>FQAMAITQKRPVYLQLVDRIKNEVATDVLSANDQLPSVRETALQEKINPNTV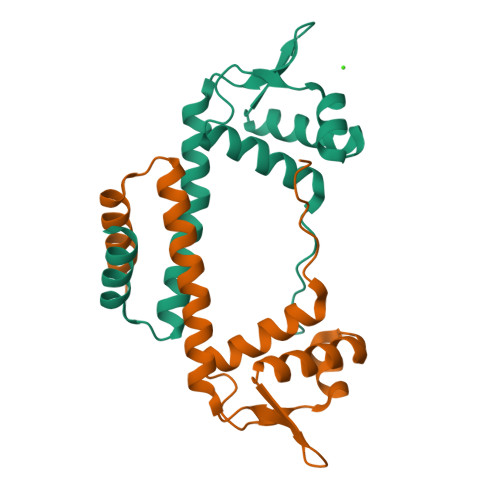AKAYKELEAQKVIRTIPGKGTFITGNTASVKNSNQNRLLADLSQVIAELIKSGVKGERIKKIVNDILGGKNAEN[5x]2-(4-bromophenyl)ethanamine 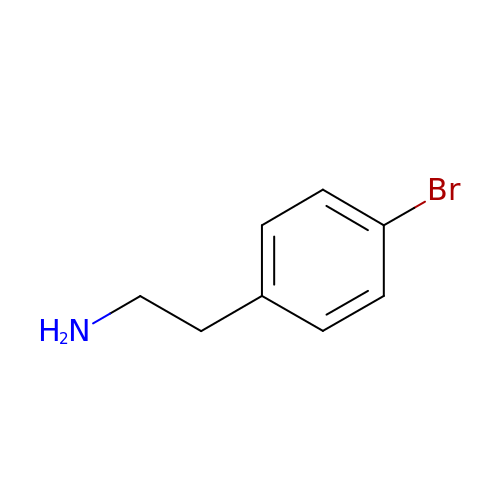| C8 H10 Br N | ZSZCXAOQVBEPME-UHFFFAOYSA-N>MTAQDITTTLLHPKGDHVLHSHAYPIFQTSTFCFDSTQQGADLFMGKGEGHIYSRLGNPTVEQFEEMVCSIEGAAGSAAFGSGMGAISSSTLAFLQKGDHLIAGDTLYGCTVSLFTHWLPRFGIEVDLIDTSDVEKVKAAWKPNTKMVYLESPANPTCKVSDIKGIAVVCHERGARLVVDATFTSPCFLKPLELGADIALHSVSKYINGHGDVIGGVSSAKTAEDIATIKFYRKDAGSLMAPMDAFLCARGMKTLPIRMQIH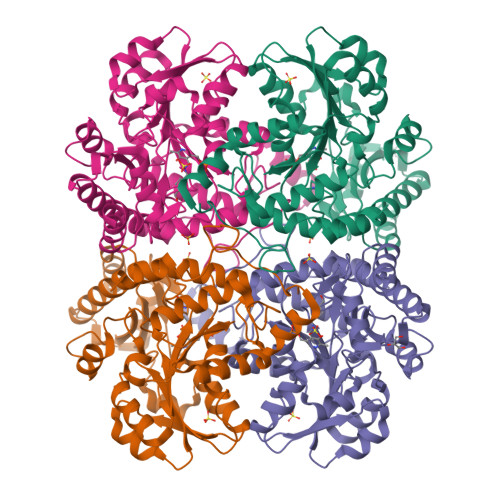MENGLKVAKFLEQHEKIVKVNHPGLESFPGHDIAKKQMTGYGSTFLFEMKSFEAAKKLMEHLKVCTLAVSLGCVDTLIEHPASMTHAAVPENIMRKQGITPELVRISVGIENVDDIIADLKQALELW[4x]> MTTNGFDPFEWRSFYFPGMSREEAHKLLGEPQVSIGTFLMRDSSRPGEYSLTVREADEGNAVCHYLIERGEPKEDGTAAAGVKIANQSFPDIPALLNHFKMRVLTEASLLAAYKKPIIEVVVGTFKFTGERETDLPFEQGERLEILSKTNQDWWEARNAL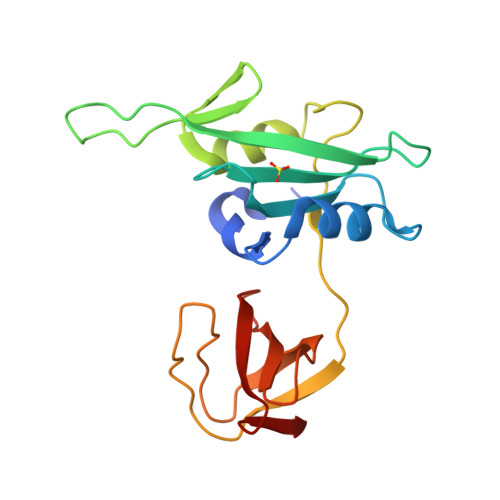GTTGLVPANYVQIQ5-(1-methylpyrazol-4-yl)-3-[1-(phenylmethyl)pyrazol-4-yl]furo[3,2-b]pyridine | C21 H17 N5 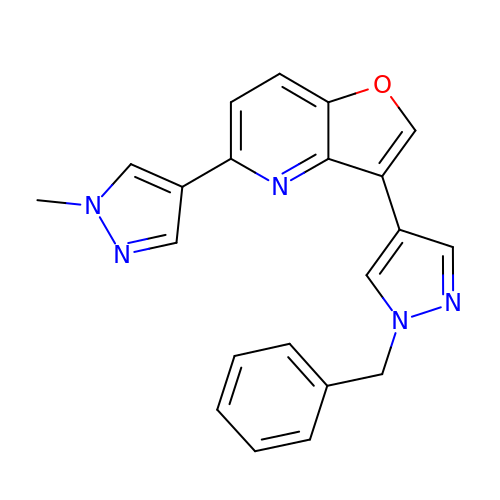O | IAJZCWZPVNGTMZ-UHFFFAOYSA-N> MGSSHHHHHHSSENLYFQGHMASMNKEMSETLTRVGPNTRMGNLLRRYWVPALMSSEIAEADGPQVRVQLLGEKLLAFRNTDGKACLISEFCSHRGVSLYFGRNEENGIRCAYHGVKFDGDGQCVDVPSSPQSCARMHIKGYPCVERGGIVWTYMGPEEHKPSPPELEWCTLPPEHVFVSKRLQYSNWLQAMEGGIDTAHVSYVHRFEVDTDPMHQGVKALDYIKADGNVKFEIEQTPFGLSLFGRRNGEPDSYYWRITQWLFPWFTLIAPFGNHALGGHVWVPIDDHNCWAWSINWQPDQPLTKEERQSMEEGKGIHVEYEEPGSFIPKANRNNDYGMDRVAQREERSYSGIFGFSAQDYSLQESMGPIQDHAAERLLPTDKAIVMARRMLNEAALGLEQGETPPALDASEQHVRPAGVLLPRDQDPVAWAREELADATKKPVFSL

Comamonas testosteroni KF1 initiates isophthalate degradation through a specialized two-component enzyme system composed of isophthalate dioxygenase (IPDO) and its cognate reductase, isophthalate dioxygenase reductase. IPDO, a Rieske oxygenase (RO), catalyzes the initial and critical dihydroxylation of isophthalate, producing cis-3,4-diol isophthalate, thereby priming the molecule for further catabolism. Rieske oxygenases form a vast enzyme class—comprising over 70,000 members—known for their chemo-, regio-, and stereoselective oxidative transformations across diverse substrates. These enzymes catalyze mono- and dioxygenation reactions through a conserved catalytic scaffold consisting of a Rieske [2Fe-2S] cluster and a mononuclear non-heme iron center. Unlike related oxygenases, phthalate dioxygenase (α3α3) and terephthalate dioxygenase (α3β3), IPDO adopts a trimer (α3) architecture, with distinct active site residues tailored to isophthalate binding.

To identify the residues involved in isophthalate recognition, we co-crystallized IPDOKF1 with its substrate and determined the structure of the isophthalate-bound complex to 3.3 Å resolution. Although the resolution was relatively low, the electron density near the mononuclear iron site clearly accommodated the isophthalate molecule, which was unambiguously modeled with a real space correlation coefficient of 0.98. The backbone conformation in the IPDOKF1-isophthalate complex structure closely resembles that of the substrate-free IPDOKF1 (RMSD 0.585 Å over 419 Cα atoms). Substrate-induced changes are localized primarily to the active site, where H257 shifts by 1.2 Å to accommodate the carboxylate group of isophthalate. The isophthalate molecule is oriented in the active site such that its C3 and C4 carbon atoms are located at 4.6 and 4.7 Å distances from the mononuclear iron, respectively, consistent with earlier reported distance between mononuclear iron of phthalate dioxygenase and phthalate. Interestingly, residues R234 and H257 participate in salt bridge interactions with the C1 and C3 carboxyl groups of isophthalate, positioned at 3.2 and 3.0 Å from R234 and H257, respectively. Additionally, the C1 carboxylate forms hydrogen bonds with the side chain hydroxyl of T175 and the main chain carbonyl of G172 at distances of 3.0 and 3.1 Å, respectively. These interactions indicate that the carboxylate groups are key for substrate anchoring within the active site. Furthermore, residues I246 and I294 contribute hydrophobic contacts, while residue F333 engages in π-π stacking interactions with the isophthalate aromatic ring. The active site architecture, particularly the positioning of polar residues, restricts isophthalate to a fixed orientation, preventing alternative binding modes.>[8x]MIYDFT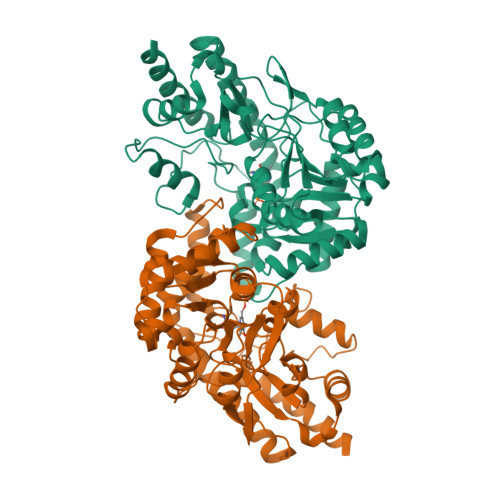TKISRKNLGSLKWDLMYSQNPEVGNEVVPLSVADMEFKNPPELIEGLKKYLDETVLGYTGPTEEYKKTVKKWMKDRHQWDIQTDWIINTAGVVPAVFNAVREFTKPGDGVIIITPVYYPFFMAIKNQERKIIECELLEKDGYYTIDFQKLEKLSKDKNNKALLFCSPHNPVGRVWKKDELQKIKDIVLKSDLMLWSDEIHFDLIMPGYEHTVFQSIDEQLADKTITFTAPSKTFNIAGMGMSNIIIKNPDIRERFTKSRDATSGMPFTTLGYKACEICYKECGKWLDGCIKVIDKNQRIVKDFFEVNHPEIKAPLIEGTYLQWIDFRALKMDHKAMEEFMIHKAQIFFDEGYIFGDGGIGFERINLAAPSSVIQESLERLNKALKDLKNRHLK> MLKIGVLVSGRGSNLQAIIDAIESGKVNASIELVISDN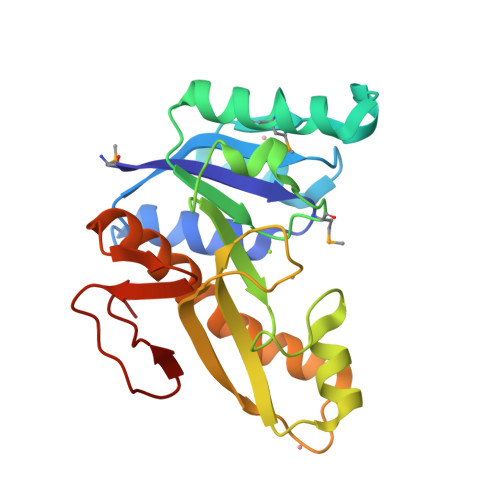PKAYAIERCKKHNVECKVIQRKEFPSKKEFEERMALELKKKGVELVVLAGFMRILSHNFLKYFPNKVINIHPSLIPAFQGLHAQKQAVEFGVKFSGCTVHIVDESVDAGPVIVQAVVPVLPEDDENTLADRILKWEHKILPQTVQWFAQDRIIIDGRKVIVKDATYGTLPVNPALEIF> GSSGSSGMDEDVLTTLKILIIGESGVGKSSLLLRFTDDTFDPELAATIGVDFKVKTISVDGNKAKLAIWDTAGQERFRTLTPSYYRGAQGVILVYDVTRRDTFVKLDNWLNELETYCTRNDIVNMLVGNKIDKENREVDRNEGLKFARKHSMLFIEASAKTCDGVQCAFEELVEKIIQ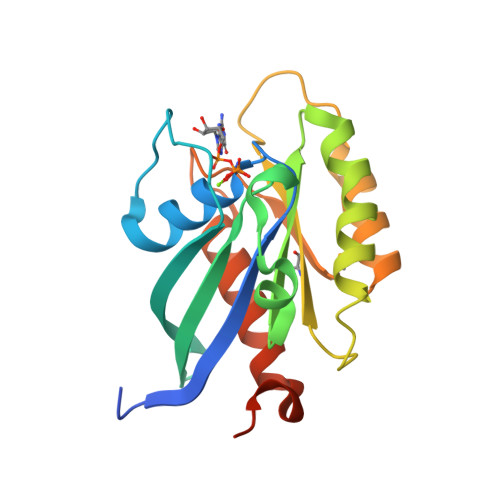TPGLWESENQNSGPSSG> YNSGKLEEFVRGNLERECIEEKCSFEEAREVFENTEKTNEFWKQYVDGDQCEPNPCLNGGLCKDDINSYECWCQVGFEGKNCELDATCNIKNGRCKQFCKTGADSKVLCSCTTGYRLAPDQKSCKPAVPFP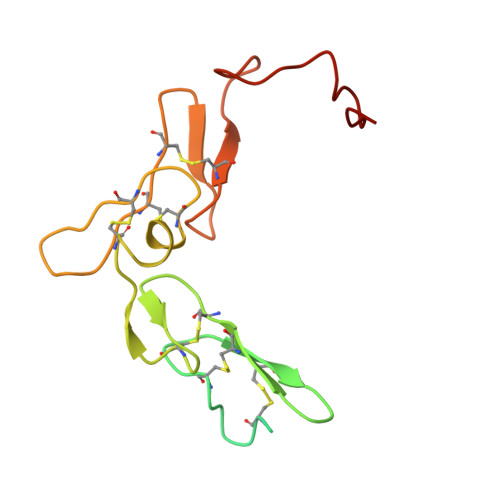CGRVSVSHSPTTLTR>DDFRVGERVWVNGNKPGFIQFLGETQFAPGQWAGIVLDEPIGKNDGSVAGVRYFQCEPLKGIFTRPSKLTRK[4x];>DSWKD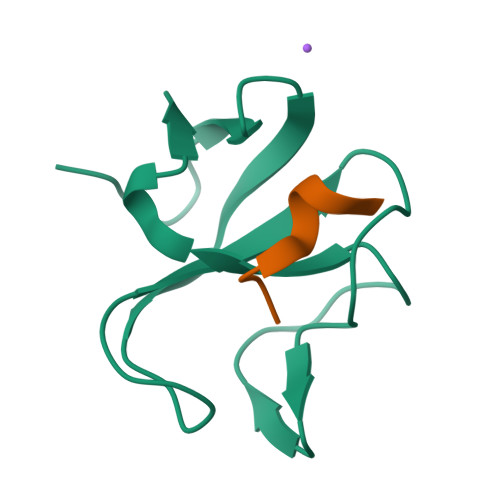GCY[4x]>GGSHDCAKVDLENAELRRKLIRTKRAFEDTYEKLRMANKAKAQVEKDIKNQIL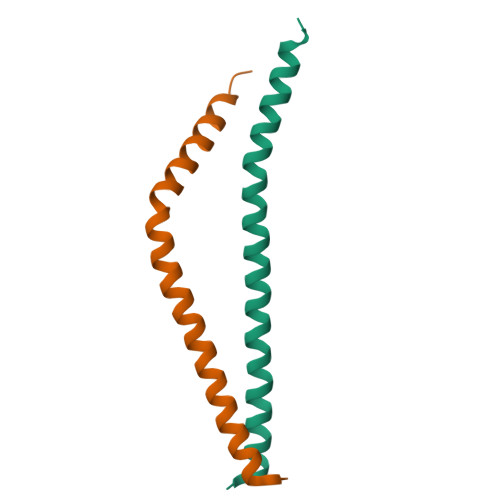KTHNVLRNVRSNMENEL[4x]> MVRLKSRYILFEIIFPPTDTNVEESVSKADILLSHHRASPADVSIKSILQEIRRSLSLNLGDYGSAKCNSLLQLKYFSN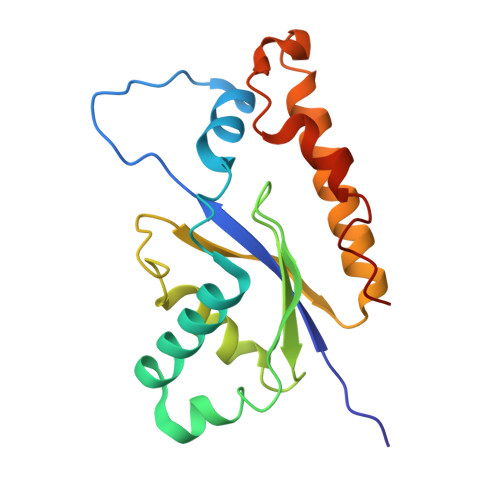KTSTGIIRCHREDCDLVIMALMLMSKIGDVDGLIVNPVKVSGTIKKIEQFAMRRNSKILNIIKCSQSSHLSDNDFIINDFKKIGRENENENEDD> AEQSSSEIKIVRDEYGMPHIYANDTWHLFYGYGYVVAQDRLFQMEMARRSTQGTVAEVLGKDFVKFDKDIRRNYWPDAIRAQIAALSPEDMSILQGYADGMN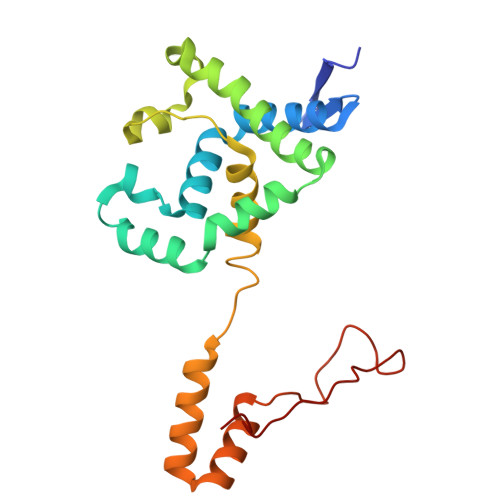AWIDKVNTNPETLLPKQFNTFGFTPKRWEPFDVAMIFVGTMANRFSDSTSEIDNLALLTALKDKYGVSQGMAVFNQLKWLVNPSAPTTIAVQESNYPLKFNQQNSQT>AGSDEVNRNECKTVVPLHTWVLISNFKLSYNILRRADGTFERDLGEYLDRRVPANARPLEGVSSFDHIIDQSVGLEVRIYRAAAEGDAEEGAAAVTRPILEFLTDAPAAEPFPVIIFFHGGSFVHSSASSTIYDSLCRRFVKLSKGVVVSVNYRRAPEHRYPCAYDDGWTALKWVMSQPFMRSGGDAQARVFLSGDSSGGNIAHHVAVRAADEGVKVCGNILLNAMFGGTERT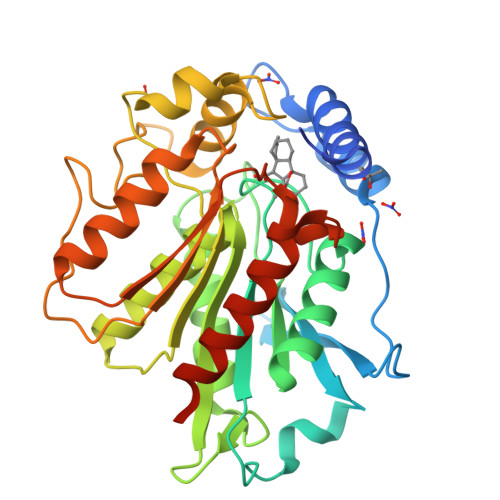ESERRLDGKYFVTLQDRDWYWKAYLPEDADRDHPACNPFGPNGRRLGGLPFAKSLIIVSGLDLTCDRQLAYADALREDGHHVKVVQCENATVGFYLLPNTVHYHEVMEEISDFLNANLYYGSHHHHHHHHHH[6x]>[22x]MSFSQAVSGLNAAATNLDVIGNNIANSATYGFKSGTASFADM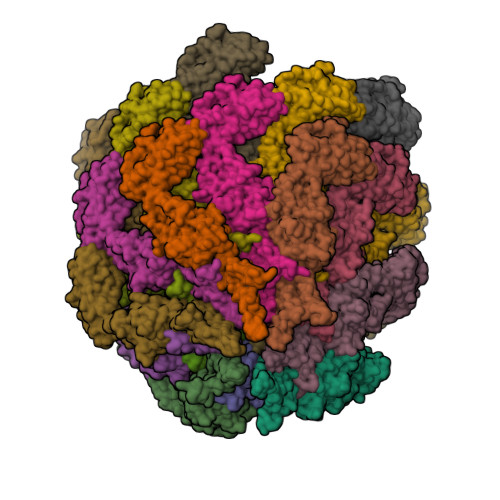FAGSKVGLGVKVAGITQDFTDGTTTNTGRGLDVAISQNGFFRLVDSNGSVFYSRNGQFKLDENRNLVNMQGMQLTGYPATGTPPTIQQGANPAPITIPNTLMAAKSTTTASMQINLNSTDPVPSKTPFSVSDADSYNKKGTVTVYDSQGNAHDMNVYFVKTKDNEWAVYTHDSSDPAATAPTTASTTLKFNENGILESGGTVNITTGTINGATAATFSLSFLNSMQQNTGANNIVATNQNGYKPGDLVSYQINNDGTVVGNYSNEQEQVLGQIVLANFANNEGLASQGDNVWAATQASGVALLGTAGSGNFGKLTNGALEASNVDLSKELVNMIVAQRNYQSNAQTIKTQDQILNTLVNLR> MDSEEVNERVKQLAEKAKEATDKEEVIEIVKELAELAKQSTDSELVNEIVKQLAEVAKEATDKELVIYIVKILAELAKQSTDSELVNEIVKQLAEVAKEATDKELVIYIVKILAELAKQSTDSELVNEIVKQLEEVAKEATDKEL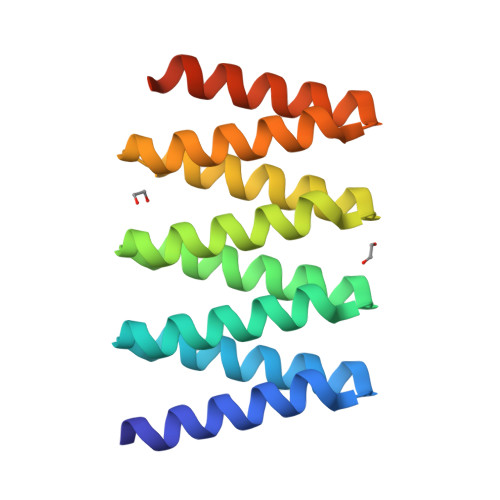VEHIEKILEELKKQSTDGWLEHHHHHH> MNLFQTVFTGSKQALAAAEGIVKQAVDEKGRDYKVAFPDTAYSLPVIFAATGKKITNVGELEGALDIVRSLIVEEEMLDKLLNSGLATAVAAEIIEAAKYVLSDAPYAEPCVGFISDPIIRSLGVPLVTGDIPGVAVILGECPDSETAAKIIKDYQSKGLLTCLVGKVIDQAIEGKVKMGLDLRVIPLGYDVTSVIHVVTIAIRAALIFGGIKGGQLNDILKYTAERVPAFVNAFGPLSELVV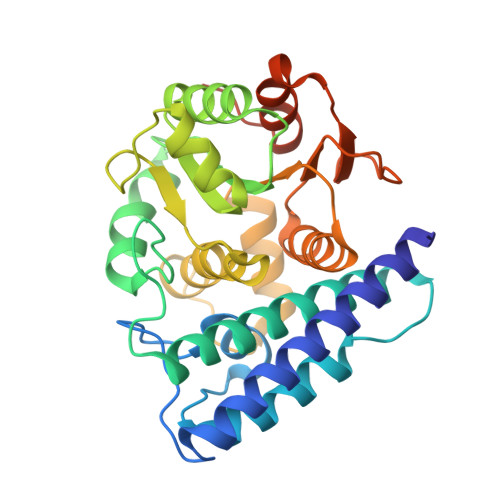SAGAGAIALGFPVLTDQVVPEVPTLLLTQKDYDKMVKTSLEARNIKIKITEIPIPVSFAAAFEGER>GSHMRYIDLRSDTVTQPTDAMRQCMLHAEVGDDVYGEDPGVNALEAYGADLLGKEAALFVPSGTMSNLLAVMSHCQRGEGAVLGSAAHIYRYEAQGSAVLGSVALQPVPMQADGSLA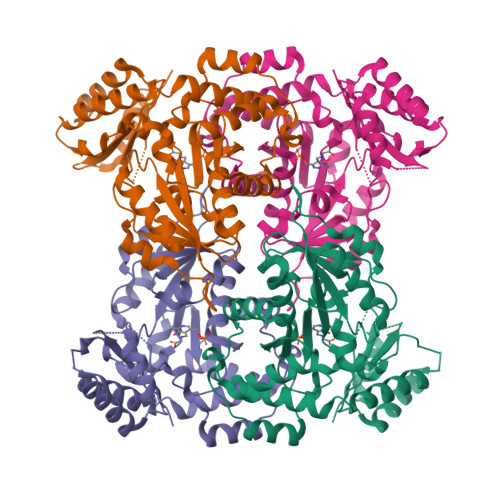LADVRAAIAPDDVYFTPTRLVCLENTHNGKVLPLPYLREMRELVDEHGLQLHLDGARLFNAVVASGHTVRELVAPFDSVSICLSKGLGAPVGSLLVGSHAFIARARRLRKMVGGGMRQAGILAQAGLFALQQHVVRLADDHRRARQLAEGLAALPGIRLDLAQVQTNMVFLQLTSGERAPLLAFMKARGILFSGYGELRLVTHLQIHDDDIEEVIDAFTEYLGA[4x]>TPEMPVLENRAAQGDITAPGGARRLTGDQTAALRDSLSDKPAKNIILLIGDGMGDSEITAARNYAEGAGGFFKGIDALPLTGQYTHYALNKKTGKPDYVTDSAASATAWSTGVKTYNGALGVDIHEKDHPTILEMAKAAGLATGNVSTAELQDATPAALVAHVTSRKCYGPSATSEKCPGNALEKGGKGSITEQLLNARADVTLGGGAKTFAETATAGEWQGKTLREQAQARGYQLVSDAASLNSVTEANQQKPLLGLFADGNMPVRWLGPKATYHGNIDKPAVTCTPNPQRNDSVPTLAQMTDKAIELLSKNEKGFFLQVEGASIDKQDHAANPCGQIGETVDLDEAVQRALEFAKKEGNTLVIVTADHAHASQIVAPDTKAPGLTQALNTKDGAVMVMSYGNSEEDSQEQ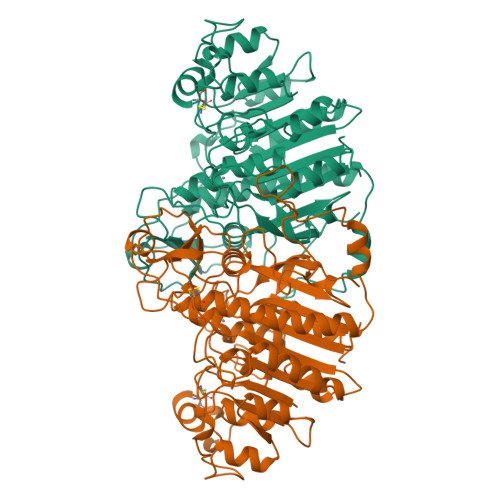TGSQLRIAAYGPHAANVVGLTDQTDLFYTMKAALGLK[2x]> MENWQATEILPKIEAPLNIFNDIKTYTAEQLFDNLRIYFGDDPSRYNISFEALLGIYCNKIEWINFFTTPIAVAANVIRFNDVSRMTLGKVLFFIQLPRVATGNDVTAPKETTIMVAKHSEKHPINISFDLSAACLEHLENTFKNTVIDQILNINALHTVLRSLKNSADSLERGLIHAFMQTLLRKSPPQFIVLTMNENKVHNKQALSRVQRSNMFQSLKNRLLTSLFFLNRNNNSSYIYRILNDMMESVTESILNDTNNYTSKENIPLDGVLLGPIGSIQKLTNILSQYISTQVVSAPISYGHFIMGKENAVTAIAYRAIMADFTQFTVNAGTEQQDTNNKSEIFDKSRAYADLKLNTLKLGDKLVAFDHLHKVYKNTDVNDPLEQSLQLTFFFPLGIYIPTETGFSTMETRVKLNDTMENNLPTSVFFHNKDQVVQRIDFADILPSVCHPIVHDSTIVERLMKNEPLPTGHRFSQLCQLKITRENPTRILQTLYNLYESRQEVPKNTNVLKNELNVEDFYKPDNPTLPTERHPFFDLTYIQKNRATEVLCTPRIMIGNMPLPLAPISFHEARTNQMLEHAKTNSHNYDFTLKIVTESLTSGSYPELAYVIEILVHGNKHAFMILKQVISQCISYWFNMKHILLFCNSFEMIMLISNHMGDELIPGAAFAHYRNLVSLIRLVKRTISISNINEQLCGEPLVNFANALFDGRLFCPFVHTMPRNDTNAKITADDTPLTQNTVRVRNYEISDVQRMNLIDSSVVFTDNDRPSNENTILSKIFYFCVLPALSNNKACGAGVNVKELVLDLFYTEPFICPDDCFQENPISSDVLMSLIREAMGPGYTVANTSSIAKQLFKSLIYINENTKILEVEVSLDPAQRHGNSVHFQSLQHILYNGLCLISPITTLRRYYQPIPFHRFFSDPGICGTMNADIQVFLNTFPHYQRNDGGFPLPPPLALEFYNWQRTPFSVYSAFCPNSLLSIMTLAAMHSKLSPVAIAIQSKSKIHPGFAATLVRTDNFDVECLLYSSRAATSIILDDPTVTAEAKDIVTTYNFTQHLSFVDMGLGFSSTTATANLKRIKSDMGSKIQNLFSAFPIHAFTNTDINTWIRHHVGIEKPNPSEGEALNIITFGGINKNPPSILLHGQQAICEVILTPVTTNINFFKLPHNPRGRESCMMGTDPHNEEAARKALYDHTQTDSDTFAATTNPWASLPGSLGDILYNTAHREQLCYNPKTYSPNAQFFTESDILKTNKMMYKVINEYCMKSNSCLNSDSEIQYSCSEGTDSFVSRPCQFLQNALPLHCSSNQALLESRSKTGNTQISETHYCNYAIGE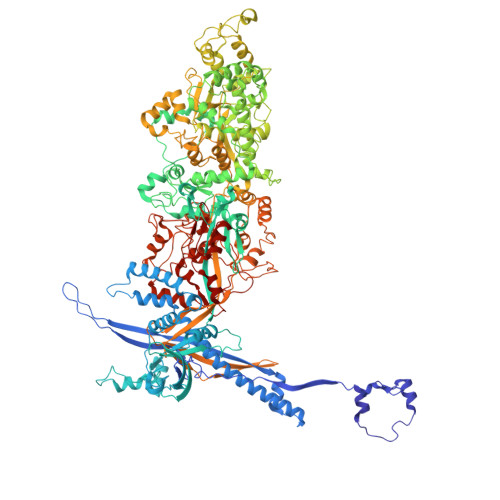TIPLQLIIESSI> GSPEFRSMTAIEDILQITTDPSDTRGYSLLKSEEVPQGSTLGVDFIDTLLLYQLTENEKLDKPFEYLNDCFRRNQQQKRITKNKPNAESLHSTFQEIDRLVIGYGVVALQIENFCMNGAFINYITGIVSNVNSYTDFLSQIIQRAILEGTALDLLNAVFPTLLEYCNKHVSHFDLNESVIYNNVLTIFELFVTFKPIAEIFTKIDGFFADYSCKPQDFERKTILGPILSLSPIEAAVAIRNYGDNLLRSKQQTAMIHESLQAEHKVVIDRLFFIVDKLVRGSLNSRTDMISYFAHIANKNHLRRADHPPFKELSSNGFMSNITLLLVRFSQPFLDISYKKIDKIDANYFNNPSLFIDLSGETRLNSDFKEADAFYDKNRKTADSKPNFISDCFFLTLTYLHYGLGGTLSFEEKMGSEIKALKEEIEKVKKIAANHDVFARFITAQLSKMEKALKTTESLRFALQGFFAHRSLQLEVFDFICGASTFLIRVVDPEHEFPFKQIKLPLIPDQIGVENVDNADFLRAHAPVPFKYYPEFVVEGPVNYSLYISKYQTSPIFRNPRLGSFVE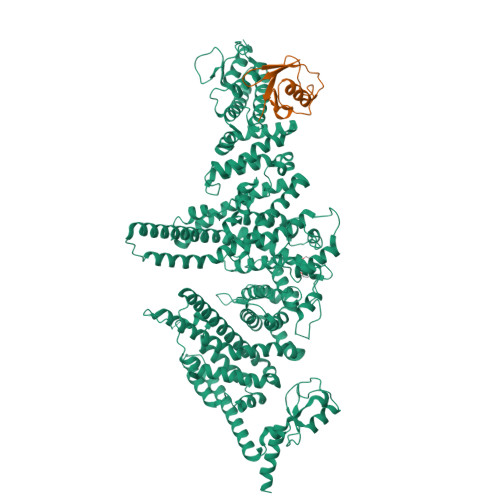FTTMVLRCPELVSNPHLKGKLVQLLSVGAMPLTDNSPGFMMDIFEHDELVNKNLLYALLDFYVIVEKTGSSSQFYDKFNSRYSISIILEELYYKIPSYKNQLIWQSQNNADFFVRFVARMLNDLTFLLDEGLSNLAEVHNIQNELDNRARGAPPTREEEDKELQTRLASASRQAKSSCGLADKSMKLFEIYSKDIPAAFVTPEIVYRLASMLNYNLESLVGPKCGELKVKDPQSYSFNPKDLLKALTTVYINLSEQSEFISAVAKDERSFNRNLFVRAVDILGRKTGLASPEFIEKLLNFANKAEEQRKADEEEDLEYGDVPDEFLDPLMYTIMKDPVILPASKMNIDRSTIKAHLLSDSTDPFNRMPLKLEDVTPNEELRQKILCFKKQKKEEAKHKASE;> MVSLTFKNFKKEKVPLDLEPSNTILETKTKLAQSISCEESQIKLIYSGKVLQDSKTVSECGLKDGDQVVFMVSQKKSTKTKVTERDPNSSSVDKLAAALEHHHHHH> MASVHGTTYELLRRQGIDTVFGNPGSNELPFLKDFPEDFRYILALQEACVVGIADGYAQASRKPAFINLHSAAGTGNAMGALSNAWNSHSPLIVTAGQQTRAMIGVEALLTNVDAANLPRPLVKWSYEPASAAEVPHAMSRAIHMASMAPQGPVYLSVPYDDWDKDADPQSHHLFDRHVSSSVRLNDQDLDILVKALNSASNPAIVLGPDVDAANANADCVMLAERLKAPVWVAPSAPRCPFPTRHPCFRGLMPAGIAAISQLLEGHDVVLVIGAPVFRYHQYDPGQYLKPGTRLISVTCDPLEAARAPMGDAIVADIGAMASALANL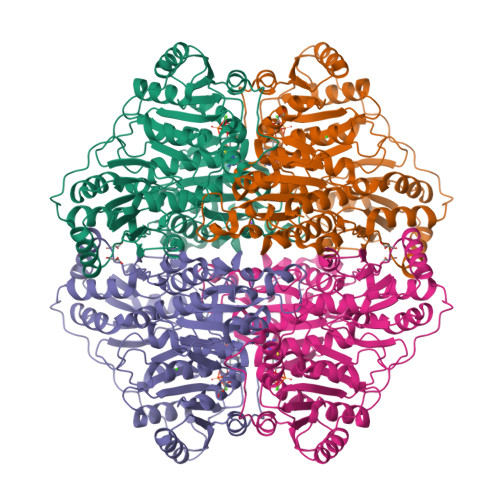VEESSRQLPTAAPEPAKVDQDAGRLHPETVFDTLNDMAPENAIYLNESTSTTAQMWQRLNMRNPGSYYFCAAGGMGFALPAAIGVQLAEPERQVIAVIGDGSANYSISALWTAAQYNIPTIFVIMNNGTYGALRWFAGVLEAENVPGLDVPGIDFRALAKGYGVQALKADNLEQLKGSLQEALSAKGPVLIEVSTVSPVKRSHHHHHH> MTIQPGTGYNNGYFYSYWNDGHGGVTYTNGPGGQFSVNWSNSGNFVGGKGWQPGTKNKVIN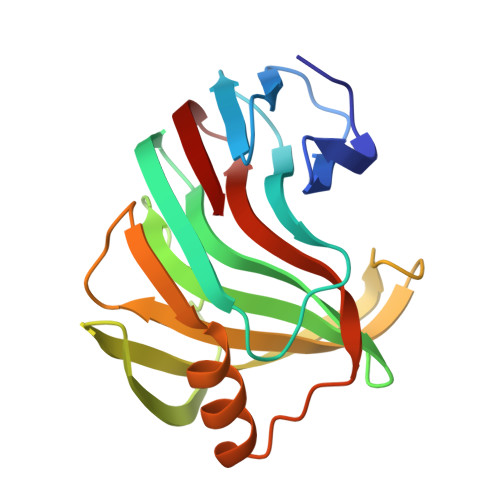FSGSYNPNGNSYLSVYGWSRNPLIEYYIVENFGTYNPSTGATKLGEVTSDGSVYDIYRTQRVNQPSIIGTATFYQYWSVRRNHRSSGSVNTANHFNAWAQQGLTLGTMDYQIVAVEGYFSSGSASITVS> LCSLDNGDC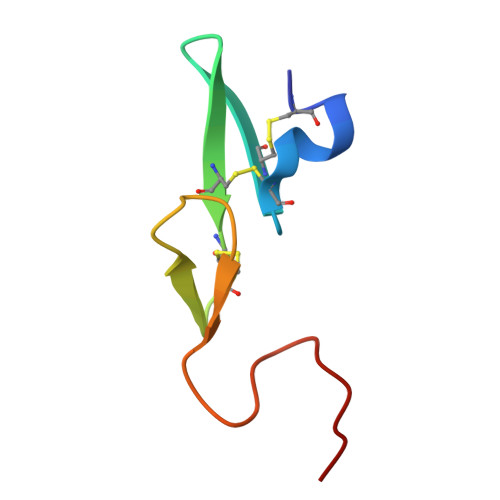DQFCHEEQNSVVCSCARGYTLADNGKACIPTGPYPCGKQTLE> GSHMASDLLELTEDMEKEISNALGHGPQDEILSSAFKLRITRGDIQTLKNYHWLNDEVINFYMNLLVERNKKQGYPALHVFSTFFYPKLKSGGYQAVKRWTKGVNLFEQEIILVPIHRKVHWSLVVIDLRKKCLKYLDSMGQKGHRICEILLQYLQDESKTKRNSDLNLLEWTHHSMKPHE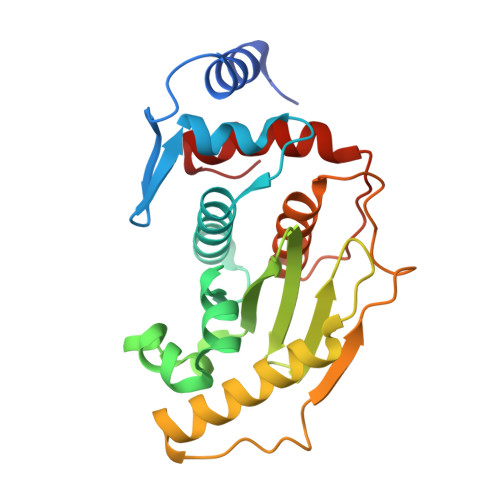IPQQLNGSDSGMFTCKYADYISRDKPITFTQHQMPLFRKKMVWEILHQQLL>KTIIINGVQFNTDEDTTILKFARDNNIDISALCFLNNCNNDINKCEICTVEVEGTGLVTACDTLIEDGMIINTNSDAVNEKIKSRISQLLDIHEFKCGPCNRRENCEFLKLVIKYKARASKPFLPKDKTEYVDERSKSLTVDRTKCLLCGRCVNACGKNTETYAMKFLNKNGKTIIGAEDEKCFDDTNCLLCGQCIIACPVAALSEKSHMDRVKNALNAPEKHVIVAMAPSVRASIGELFNMGFGVDVTGKIYTALRQLGFDKIFDINFGADMTIMEAATELVQRIENNGPFPMFTSCCPGWVRQAENYYPELLNNLSSAKSPQQIFGTASKTYYPSISGLDPKNVFTVTVMPCTSKKFEADRPQMEKDGLRDIDAVITTRELAKMIKDAKIPFAKLEDSEADPAMGEYSGAGAIFGATGGVMEAALRSAKDFAENAELEDIEYKQVRGLNGIKEAEVEINNNKYNVAVINGASNLFKFMKSGMINEKQYHFIEVMACHGGCVNGGGQPHVNPKDLEKVDIKKVRASVLYNQDEHLSKRKSHENTALVKMYQNYFGKPGEGRAHEILHFKYKKSAWSHPQFEK[2x]

Hydrogen (H2) turnover in [FeFe]-hydrogenases is proposed to occur at the distal iron site (Fed) of the [2Fe2S] moiety (2FeH), which is part of the H-cluster1. The distal iron ion exchanges protons with a conserved proton-transfer pathway (PTP)23 via an azadithiolate ligand (adt) that bridges both iron sites. The binuclear metal cofactors of [FeFe]- and [NiFe]-hydrogenases have been suggested to oxidize H2 by enhancing the acidity of H2 in the presence of a base, thus facilitating its heterolytic cleavage into a proton (H+) and hydride (H−) as a first intermediate step. According to the current working model for the catalytic mechanism of [FeFe]-hydrogenases, binding of H2 to the oxidized active ready state (Hox) results in the heterolytic cleavage of H2, with Hhyd as the first intermediate.

To verify that an interference with the PTP enhances the population of the Hhyd state under H2 exposure, we blocked the PTP in HydA1 and CpI via site-directed mutagenesis at two strictly conserved positions for each protein. Position 1 (C169 of HydA1/C299 of CpI), which was shown in earlier experimental data to be involved in catalytic proton transfer, marks the most proximal position of the PTP to the 2FeH sub-cluster, while position 2 (E141 of HydA1/E279 of CpI) is situated more distant from the H-cluster. An exchange to alanine almost completely abolished H2-release activity for all variants. To probe the structural integrity and unequivocally connect the monitored effects to an interrupted PTP, we solved the crystal structure of CpI E279A. The X-ray structure illustrates a fully intact H-cluster and overall identical structural features compared to wild-type CpI, with the exception of the clearly diminished electron density at position 279, which is in full accordance with an exchange from glutamate to alanine. As a consequence of this non-conservative exchange, the path of polar side chains is interrupted between S319 and the harnessed H2O molecule. Figure 4a,b shows the reaction of enzyme variants C169A of HydA1 and E279A of CpI towards H2 (black graph) at pH 8. Similar to the effect of acidification or sample drying, the oxidized state is lost in favour of bands at 1,978/1,962/1,863 cm−1 or 1,985/1,970/1,858 cm−1, respectively. When switching the purging gas from H2 to D2, CpI E279A and HydA1 C169A showed a selective shift to lower energies by 5–6 cm−1 of the band at 1,860 cm−1, which corresponds to the stretching vibration of μCO. In return, the analogous behaviour of cysteine and glutamate variants provides experimental proof for the involvement of the median glutamic acid residue (E141HydA1/E279CpI) in the proton-transfer mechanism of [FeFe]-hydrogenases.> MAEYPLPKFHFQVDWGGSRLGFTEVSGLDVETEVIEYREGNLPQY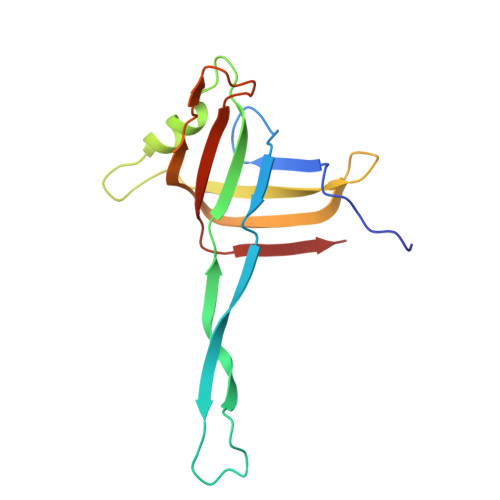HKLKMPGMQKFSNITMKRGTFQGDNDFYKWWNTVALNTIERRDLTISLLNEKHEPVVVWKVNRAWPTKVQSTDLKGDGNEVAIESIEVAHEGLTIQNG>MLSSTKEYLQALRDGKYLLFLQWPKFIAEYYGKSDKNQEADEMVSLLIFEWLNNGFCLDDIKKFAILYAVHEMESRPLREGLSYALTTISIALFPCMVYLTNNLQEHYITSKKLSSKEVLQLMTMNNAYLEKQRFVEFLGQEQDKFFTWVKEADSSAVSKAFDQIYSVTYLKYLIEDYLSLLESAHLPTDQLKSSRISLVVRLAKYLHEQTELTQDVHDEIAVYVKKLWEMQPAEFEEEFLKKISPLPFIDNTVRILTGLSARFFSILQPPSPPLNINSDTDKNPKV[4x]

Lpg0393 is a newly identified Legionella effector classified as a hypothetical protein. Through X-ray crystallographic analysis, we show that Lpg0393 contains a Vps9-like domain, which is structurally most similar to the catalytic core of human Rabex-5 that activates the endosomal Rab proteins Rab5, Rab21 and Rab22. Consistently, Lpg0393 exhibited a guanine-nucleotide exchange factor activity toward the endosomal Rabs. This work identifies the first example of a bacterial guanine-nucleotide exchange factor that is active towards the Rab5 sub-cluster members, implying that the activation of these Rab proteins might be advantageous for the intracellular survival of Legionella.

We subsequently prepared a construct having a deletion of the C-terminal 17 residue segment, which was predicted to have an unstructured random coil conformation. This construct, which is referred to as Lpg0393Δ17, was crystallized and its crystal structure was determined by the single wavelength anomalous dispersion method. Lpg0393Δ17 adopts an all α-helical tertiary structure containing 12 α-helices that are arranged to form two physically distinct domains. The N-terminal domain contains seven α-helices and makes roughly a 90° angle with the C-terminal domain that forms a helical bundle structure. The asymmetric unit of the crystal contained four molecules of Lpg0393Δ17 that formed two homodimer-like pairs, mainly through the association between two C-terminal domains. Probably due to fairly extensive intermolecular interactions, the conformations of the two C-terminal helices, α11 and α12, are different between the two Lpg0393Δ17 molecules involved in the dimer formation. In one molecule, α11 and α12 are parallel with each other and separated by a short two-residue loop, and in the other molecule, α11 and α12 make a ∼70° angle to form a wedge-like interface with which α12 of the first molecule interacts. In contrast with the crystallographic observation, Lpg0393Δ17 was eluted from a gel-filtration column, with a deduced molecular weight of 35 kDa, close to the calculated monomeric size of the protein (31.5 kDa), and suggesting that the physiological state of the protein is monomeric. Remarkably, the domain organization of Rabex-5 is reversed in comparison with that of Lpg0393Δ17, which comprises the N-terminal Vps9-like domain followed by the C-terminal helix bundle. Notably, as predicted by the initial bioinformatics, Asp313 and Tyr354 of Rabex-5 are conserved as Asp41 and Tyr84 in the Vps9-like domain of Lpg0393.>[2x]TFGTFQDAYLSQLRDIYHS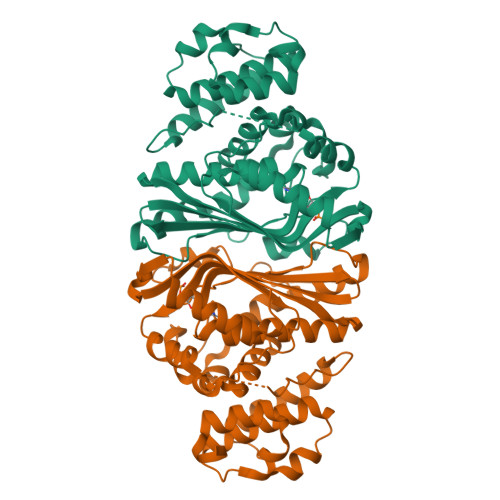PEFRNAPRGQASRERIGAGFRLLDPVQRHISVPARRANVVFNFAEALWYLSGSDRLDFIQYYAPGIAAYSADGRTLRGTAYGPRIFRHPAGGVNQWENVVKTLTDDPDSKRAVIQIFDPRELAVADNIDVACTLALQFLIRDGLLCGIGYMRANDAFRGAVSDVFSFTFLQEFTARYLGLGIGTYHHVVGSVHIYDSDARWAERVLDAATPDGGPRPGFPAMPDGDNWPHVRRVLEWEERLRTNAARLSADALDALDLPAYWKHVVALFEAHRQVRHEDTPDRALLAALPEVYRQSLAVKWPGHFG>[2x]MQGCPFAKRDGTVDSSLPQKRADAPETTTFGRCAVKSNQAGGGTRSHDWWPCQLRLDVLRQFQPSQNPLGGDFDYAEAFQSLDYEAVKKDIAALMTESQDWWPADFGNYGGLFVRMAWHSAGTYRAMDGRGGGGMGQQRFAPLN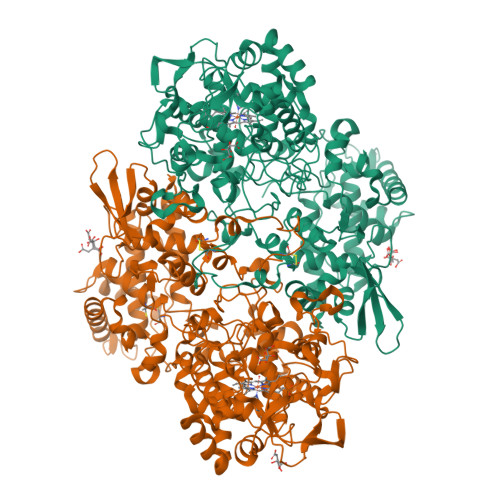SWPDNQNLDKARRLIWPIKQKYGNKISWADLMLLTGNVALENMGFKTLGFGGGRADTWQSDEAVYWGAETTFVPQGNDVRYNNSVDINARADKLEKPLAATHMGLIYVNPEGPNGTPDPAASAKDIREAFGRMGMNDTETVALIAGGHAFGKTHGAVKGSNIGPAPEAADLGMQGLGWHNSVGDGNGPNQMTSGLEVIWTKTPTKWSNGYLESLINNNWTLVESPAGAHQWEAVNGTVDYPDPFDKTKFRKATMLTSDLALINDPEYLKISQRWLEHPEELADAFAKAWFKLLHRDLGPTTRYLGPEVPKESFIWQDPLPAREGDLIDDADVDKLKAAILSTDGLDVSKLASTAMACATTYRNSDKRGGCNGARIALEPQRNWVSNNPTQLSAVLDALKKVQSDFNGSNGNKKVSLADLIVLGGTAAVEKAAKDAGVDIKVPFSAGRVDATQEQTDVTQFSYLEPQADGFRNYGRGTARARTEEIMVDKASQLTLTPPELTVLVGGMRALGANYDGSDVGVFTANKGKLTPDFFVNLVDMNIAWTASGADGESWVGTDRKSRSEKYKGSRADLVFGSHAELRAIAEVYAENGNQEKFVKDFVAAWTKVMNLDRFDLKVKK Orf virus, a member of the parapoxviridae, encodes for the Bcl-2 homolog ORFV125, a potent inhibitor of Bcl-2-mediated apoptosis in the host. ORFV125 acts by directly engaging host proapoptotic Bcl-2 proteins including Bak and Bax as well as the BH3-only proteins Hrk and Puma. ORFV125 adopts the conserved Bcl-2 fold with seven α-helices in a domain-swapped dimeric configuration where the α1 helix of one protomer is swapped with the neighbouring protomer to form the dimer interface as previously seen in other poxvirus genera such as VACV F1L, VARV F1L, DPV022 and TANV16L. An Arg located in the structurally equivalent BH1 region of ORFV125 forms an ionic interaction with the conserved Asp in the BH3 motif in a manner that mimics the canonical ionic interaction seen in host Bcl-2:BH3 motif complexes.

For ORFV125:Puma BH3 complex a clear and continuous electron density map was observed for ORFV125 residues 5–61 and 65–133, and Puma BH3 motif residues 132–155, with the remainder of the residues presumed to be disordered. Puma BH3 is bound to ORFV125 via the canonical hydrophobic ligand binding groove that is formed by helices α2–α5. The four canonical BH3 motif defining residues from Puma, I137, L141 and M144 and L148, engage four hydrophobic pockets of the canonical ORFV125 ligand binding groove. Furthermore, Puma Y152 occupies a fifth hydrophobic pocket in ORFV125, which is formed by residues A39, V42, W133 and V137. The hallmark of pro-survival Bcl-2 interactions with BH3 motifs is the presence of an ionic interaction between pro-survival Bcl-2 proteins and pro-apoptotic BH3 motif ligands between a conserved arginine in the BH1 motif and aspartate of the BH3-motif. In ORFV125:Puma this interaction is formed between R87ORFV125 and D146Puma. An additional ionic interaction was observed between E80ORFV125 and R142Puma, and this interaction is supplemented by hydrogen bonds between E54ORFV125 and Q140Puma as well as between G86ORFV125 and N149Puma. A comparison of ORFV125:Puma BH3 complex with TANV16L: Puma BH3 reveals that the mode of interaction is nearly identical, despite the ORFV125:Puma interaction being approximately four-fold lower in affinity. However, in ORFV:Puma BH3 a fifth hydrophobic pocket is used by residue Y152PUMA, a feature that has been previously observed for Bax complexes of Mcl-1, Bcl-xL and Bcl-2, where Bax M74 is lodged in a comparable pocket. In contrast to Q140PUMA, R142PUMA formed an additional ionic interaction with E80ORFV125 that is not seen in TANV16L:Puma BH3 complex.

>[2x]GPLGSMANRDDIDASAVMAAYLAREYAEAVEEQLTPRERDALEALRVSGEEVRSPLLQELSNAGEHRANPENSHIPAALVSALLEAPTSPGRMVTAVELCAQMGRLWTRGRQLVDFMRLVYVLLDRLPPTADEDLGAWLQAVARVHGT;>EEQWAREIGAQLRRMADDLNAQYERR[2x]> AVPFVEDWDLVQTL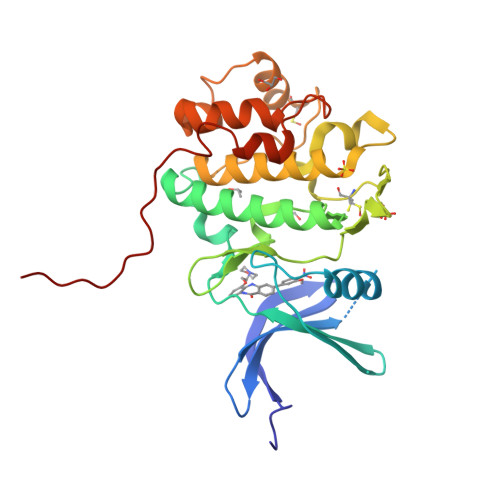GEGAYGEVQLAVNRVTEEAVAVKIVDMKRAVDCPENIKKEICINKMLNHENVVKFYGHRREGNIQYLFLEYCSGGELFDRIEPDIGMPEPDAQRFFHQLMAGVVYLHGIGITHRDIKPENLLLDERDNLKISDFGLATVFRYNNRERLLNKMCGTLPYVAPELLKRREFHAEPVDVWSCGIVLTAMLAGELPWDQPSDSCQEYSDWKEKKTYLNPWKKIDSAPLALLHKILVENPSARITIPDIKKDRWYNKPLKKGAKRPRVTS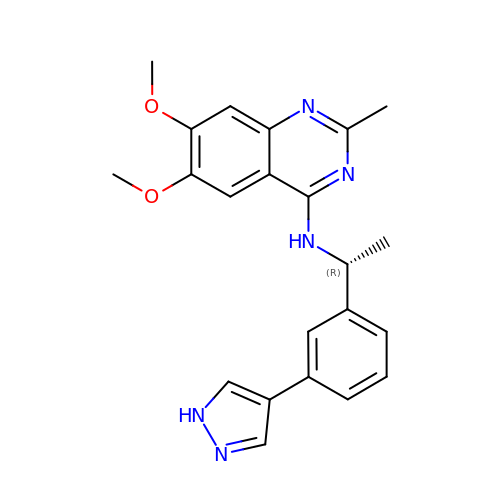6,7-dimethoxy-2-methyl-~{N}-[(1~{R})-1-[3-(1~{H}-pyrazol-4-yl)phenyl]ethyl]quinazolin-4-amine | C22 H23 N5 O2 | OYHDNGCDWWAYLR-CYBMUJFWSA-N> MQHDLFEHDPAIRQLIGHIDNIPAPELESRWPRSVVDLIDVLENELKRQNVSNPRELARKQAVALSCFLGGRQFYIPCGDTILTALRDDLLYCQFNGRNMEELRRQYRLSQPQIYQIIARQRKLHTRR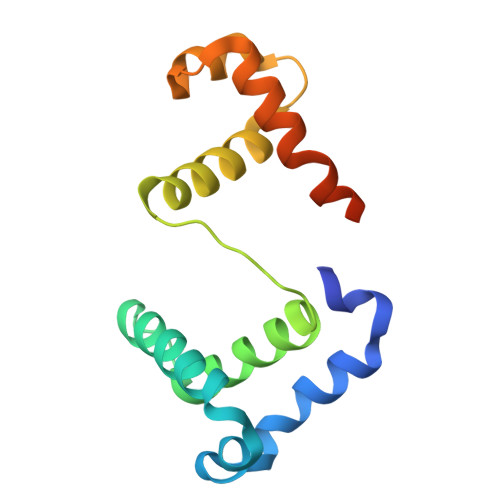HQPDLFSPETPK>GAMALPSGSDPAFSQPKSVLDAGLTCQGASPSSVSKPILLVPGTGTTGPQSFDSNWIPLSAQLGYTPCWISPPPFMLNDTQVNTEYMVNAITTLYAGSGNNKLPVLTVCQGGLVAQWGLTFFPSIRSKVDRLMAFAPDYKGTVLAGPLDALAGSAPSVWQQTTGSALTTALRNAGGLTQIVPTTNLYSATDEIVQPQVSNSPLDSSYLFNGKNVQAQAVCGPLFVIDHAGSLTSQFSYVVGRSALRSTTGQARSADYGITDCNPLPANDLTPEQKVAAAALLAPYYAAIVAGPKQNCE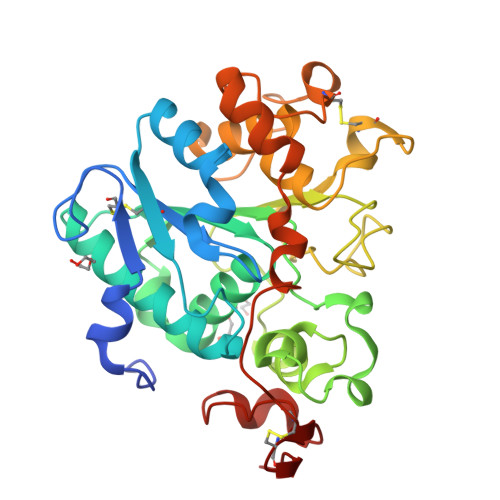PDLMPYARPFAVGKRTCSGIVTP[2x]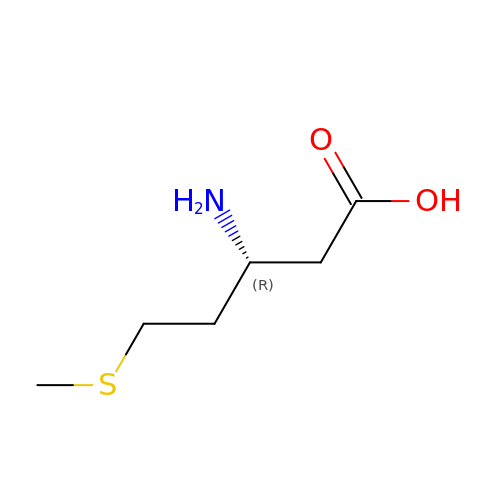(3R)-3-amino-5-(methylsulfanyl)pentanoic acid | C6 H13 N O2 S | QWVNCDVONVDGDV-YFKPBYRVSA-N>[3x]TEGSSKPRVAVTTSFLNDMVYQLAGDEVERDLLIPAGEDPHLYVAKSSDLSKLQKADLVLYHGLHFEGKMVEALEKTGVAVSKNFNAKDLNTMDEDGEEIVDPHFWFSIPLYKSAVAVASEELQKLLPAKAEMIQKNTEKYQAQLDDLHAWVEKELSVIPKESRYLVTPHDAFNYFAASYDFTLYAPQGVSTDSEVANSDMIETVNLIIDHNIKAIFTESTTNPERMKKLQEAVKAKGGQVEVVTGEGKELFSDSLAPEGEEGDTFIDMYKHNVKLMVKYLK

TroA is a substrate binding protein for uptake of multiple metal ions. The overall structure of SsTroA is typical of SBPs in the A-1 family. The peptide chain crosses between the N-terminal and C-terminal domains only once linking the two (β/α)4 domains via a 33-residue kinked rigid α-helical backbone that runs the full length of the molecule and the metal binding site is buried in the interdomain interface. Taken together, the structural and functional data we have presented here clearly demonstrate that SsTroA binds both Zn2+ and Mn2+ with high affinity.

To obtain further insight into the function of SsTroA, we determined the X-ray crystal structure of the Zn2+-bound form of the SsTroA at a resolution of 2.6 Å, and further characterized the recombinant SsTroA. The final structure was refined to a resolution of 2.6 Å and consists of 278 amino acids (residues 40–317). In our structure, we clearly observed the metal binding pocket provided by the buried surface between the N-terminal and C-terminal domains. Independent experimental evidence has demonstrated that the ion bound in the metal binding pocket of recombinant SsTroA is Zn2+ (see metal content analysis). Zinc is pentacoordinated by His 76 (bond length, 2.14 Å), His 139 (2.11 Å), His 205 (2.18 Å) and Asp 289 (2.20 Å, 2.38 Å). His 76 and His 139 are provided by the N-terminal domain, while His 205 and Asp 289 are contributed by the C-terminal domain. The Zn coordination in our structure is best described as distorted square pyramidal. The binding site is buried ∼7 Å below the molecule surface and the four coordinating residues are also completely buried. Accordingly, our structure indicated that Mn2+ is likely to be the natural ligand. Intriguingly, in the structure of SsTroA, we observed two distinctive flexible loops mainly composed of charged residues, and these two flexible loops were designated as Loop 1 (Asn 126-Pro 38) and Loop 2 (Tyr 279-Glu 285).>[2x]MAKKTLPAGVKSPPYIFSPIPFLGHAIAFGKSPIEFLENAYEKYGPVFSFTMVGKTFTYLLGSDAAALLFNSKNEDLNAEDVYSRLTTPVFGKGVAYDVPNPVFLEQKKMLKSGLNIAHFKQHVSIIEKETKEYFESWGESGEKNVFEALSELIILTASHCLHGKEIRSQLNEKVAQLYADLDGGFSHAAWLLPGWLPLPSFRRRDRAHREIKDIFYKAIQKRRQSQE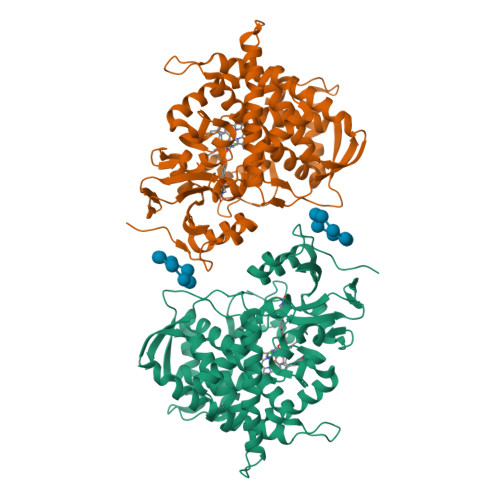KIDDILQTLLDATYKDGRPLTDDEVAGMLIGLLLAGQHTSSTTSAWMGFFLARDKTLQKKCYLEQKTVCGENLPPLTYDQLKDLNLLDRCIKETLRLRPPIMIMMRMARTPQTVAGYTIPPGHQVCVSPTVNQRLKDSWVERLDFNPDRYLQDNPASGEKFAYVPFGAGRHRCIGENFAYVQIKTIWSTMLRLYEFDLIDGYFPTVNYTTMIHTPENPVIRYKRRSTHHHHHH>MTDISQMYDQLSDPFAGLGAGNIHLGYFDGPDDAATLAEAADRLTDQLIARLPVVRDHRVLDVGCGVGK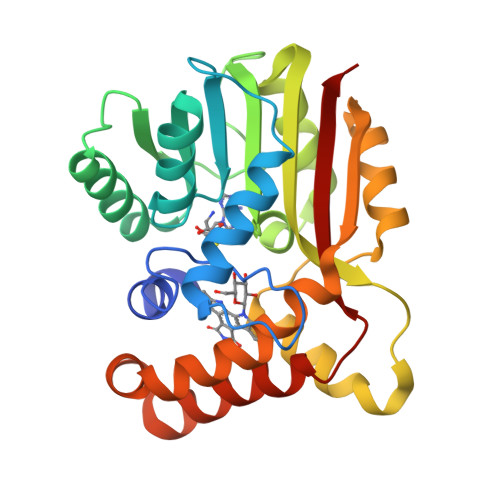PALRLAGDLGVRVVGVSISEAQIGIANEAARAAGLADRVSFRYADAMRLPFPDASFDGVWAMESLHHMPDRLQALREIARVLRHGGVLSIADFVQLGPVREQDEEALRAFRSGGGVHTLTGIAEYEAEIADAGLTLTSSSDISANVRPSMVRTAEAIRGAADAFLPLMGEEGLRRLIDNFERAATVPQIGYALFAARRS[3x]Monothiophosphate | H3 O3 P S | 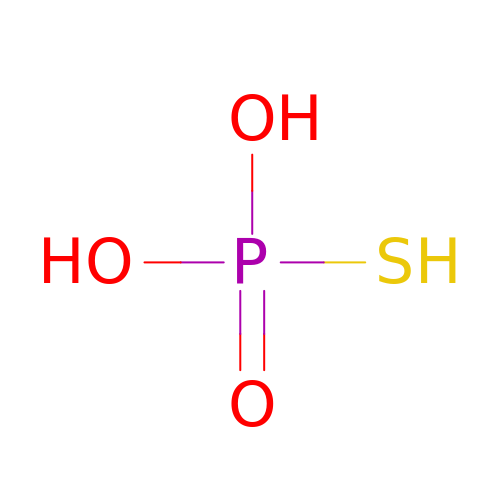RYYWUUFWQRZTIU-UHFFFAOYSA-N Pro‐apoptotic (or executioner) proteins such as BAK and BAX activate apoptosis through pore formation in the mitochondrial membrane; anti‐apoptotic proteins including BCL‐2, MCL‐1 and BCL‐xL, sequester pro‐apoptotic members to prevent cell death; and a group of regulatory proteins which bind to other BCL‐2 members (including BIM, BID, BAD, NOXA and PUMA), mediate initiation of apoptosis. In all cases binding between BCL‐2 family members occurs through the BH3 homology domain of one protein, which forms an α‐helix upon binding and docks into a complementary cleft on its partner. We have used phage display to isolate Affimer reagents (non‐antibody‐binding proteins based on a conserved scaffold) to identify ligands for MCL‐1, BCL‐xL, BCL‐2, BAK and BAX, then used multiple biophysical characterisation methods to probe the interactions. Co‐crystal structures reveal an unprecedented mode of molecular recognition; where a BH3 helix is normally bound, flexible loops from the Affimer dock into the BH3 binding cleft.

BCL‐xL‐AF10 showed problems during purification so was not further characterised. Both BCL‐xL‐AF6 (IC50=448±53 nM) and BCL‐xL‐AF7 (IC50=393 ±54 nM) were shown to act as sub μM inhibitors of the BCL‐xL/BAK interaction but were ineffective in inhibiting the MCL‐1/NOXA−B interaction. In the case of BCL‐xL‐AF6 a particularly strong enthalpic contribution was observed. For BCL‐xL‐AF6/BCL‐xL, the crystals diffracted to 1.91 Å, and the asymmetric unit contains one domain swapped dimer of BCL‐xL, with one BCL‐xL‐AF6 bound to the cleft of each monomer. The residues within the VRs of both Affimers interact with residues lining the BH3‐binding cleft on the surface of BCL‐xL. However, the universally conserved BH3 Asp which hydrogen‐bonds to Arg on BCL2‐ family members is not replicated in any way by the Affimer. On inspection it is apparent that the Affimers select a distinct conformation of the BCL‐xL domain. The binding groove on BCL‐xL is formed by helices 3 and 4 and helix 3 is mobile such that the width of the groove can vary. When BH3 peptide is bound, helix 3 moves to accommodate the peptide in a relatively wide groove (groove open conformation). When bound to BAK peptide the groove is 14.8 Å wide at the widest point, whereas in the small molecule and Affimer bound conformation it is ∼11.0 Å wide. In this case, not only does the Affimer bound conformation correspond to a small molecule bound conformation (thus this might conceptually be a better starting point for structure based drug design), but the groove closed conformation is also a conformation where the groove is too narrow to accommodate the BH3 helix, possibly potentiating the orthosteric competitive effect.

>[2x]MSQSNRELVVDFLSYKLSQKGYSWSQMAAVKQALREAGDEFELRYRRAFSDLTSQLHITPGTAYQSFEQVVNELFRDGVNWGRIVAFFSFGGALCVESVDKEMQVLVSRIAAWMATYLNDHLEPWIQENGGWDTFVELYGNNAAAESRKGQER;>[2x]SENSLEIEELARFAVDEHNKKENALLEFVRVVKAKEQERNSIFEEFTMYYLTLEAKDGGKKKLYEAKVWVKRDLVFGGPENFKELQEFKPV>DALKPEDKVKFRQASYTTMAWNMGKIKAMVVDGTMPFSQTQVSAAANVIAAIANSGMGALYSPDTLGVVGFKKSRLKENFFQEQDEVRKIATNFVEQANKLAEVAAMGDKDEIKAQF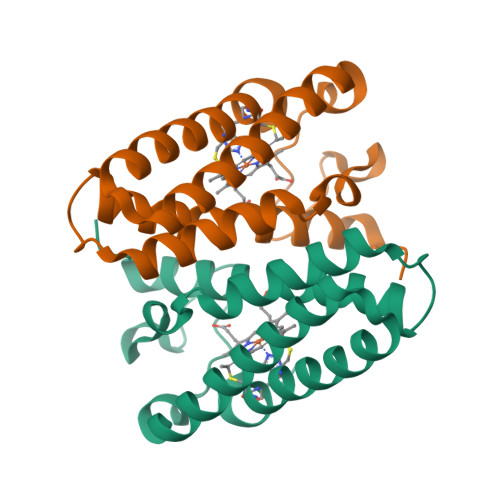GEVGKACKACHEKFREEE[4x]A prototype of a Gram-negative epsilon/zeta TA module, the epsilon_1/zeta_1 (ngε_1/ngζ_1) TA system, is encoded by Neisseria gonorrhoeae, an obligate human pathogen causing the sexually transmitted disease gonorrhoea. Thereby, we identified a yet undescribed enzymatic activity. This proteobacterial zeta toxin phosphorylates UDP-activated sugar species at the C4′-OH group of the hexose moiety which eventually causes a lytic phenotype. The toxic activity is inhibited by co-expression of ngε_1 antitoxin, corroborating that the ngε_1 / ngζ_1 locus encodes for a toxin/antitoxin pair. As expected for a bona-fide type II TA system, we demonstrated protein-protein complex formation between ngε_1 and ngζ_1, which assemble into a heterodimeric complex.

To this end, we first determined the crystal structure of the catalytically inactive ngε_1/ngζ_1(K115A) selenomethionine substituted protein complex at 2.4 Å resolution using single anomalous dispersion experiments. We found four heterodimeric ngε_1/ngζ_1(K115A) TA complex molecules located in the asymmetric unit, a complex arrangement which we also observed in solution. In fact, not only the quaternary structure is set apart from known zeta toxins, but also the tertiary structure and mode of inhibition is very different to other zeta toxins. Strikingly ngε_1 binds as an extended polypeptide stretch onto the molecular surface of ngζ_1 and does not fold into a globular domain. Furthermore, the C-terminal part of the first helix, the second helix and the connecting loop region of ngε_1 cover the potential ATP binding site. In addition, also the tertiary structure of ngζ_1 is different to known zeta toxins, as it consists of two domains. Although our initial analysis of the primary sequence did not identify these homologues, a structural alignment revealed that two sequence blocks were shuffled by swapping position within the polypeptide chain. Yet, two loop regions were topologically rewired in ngζ_1 when compared with other zeta toxins leading to a similar tertiary structure albeit these two blocks occur at different position within the amino acid sequence. Nevertheless, residues that have previously been shown to be important for enzyme catalysis are found to be structurally conserved in ngζ_1. Finally, the C-terminal domain has the fold of an oligonucleotide/oligosaccharide binding domain (OB-domain) and consists of a five-stranded Greek-key β-barrel that is in an open distorted conformation capped by a short α-helix.

>MNKVEPQESNAIRMIKEACEKNRRMMTDEAFRKEVEKRLYAGPSPELLAKLRVLWAANKEQ[4x];>[4x]MVKLSSDINLRDFGNNEYLSSVQDEAIRFATEQTDEILSLYSQHADTEGGRYVCADTFKELFPAFENKEDRATVNNAIHNSAAVLSSTQFDEVLKRDEPQKKEVIFVTGIPGSGATSTVKNMMMQDTTKLLFEGQLARPQSAFRKIEQCLERNLEVTIVAVSMRAERASDNTYKRFNEYGRGASIGIMADIQANLPDGLKQIRDKFGDAVKIVGINQDRNSEFIDKFDDVIKMLSLGSQEQILGRLAEKIQSDFDSGKISRECFNQAKGSMDLESVFAKKEYSQQRVVTNSKGVTLETKSANELWSKVEQIPVTGMKAGIYLLGQAKKAETGQTYSGEIIYKDAAAVFQKTKNGLVRHNATHNEERLAKLVEIGQNVSIGSNKGKLIVKSLEYSAKKSISR> MYARFRTRSKFYFRPARPALAYNVDPNVMRRPKVKRGLLKGTYSDETVDLRDRERLELLESMRHPRERDFYQDHTYHNQWLRRDLEKHQKQQLAARYKYFAPDFEISPWIWYPGDIVEVVSGEGIGQRGTIIAVIKYKNEIVVQNINVQ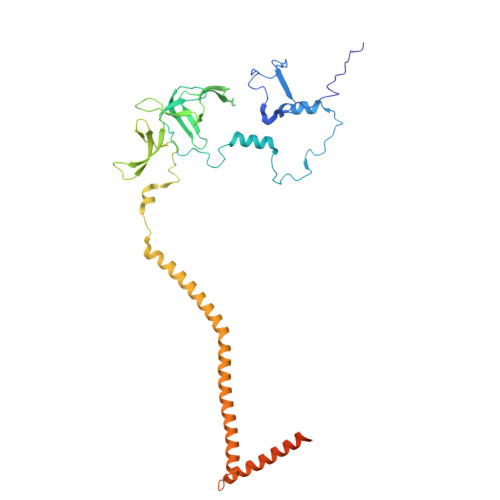DVVIPASESRPEQIVQREHPISVTRVRHVDPSTNEICNIEMVKVRNKETGEMEEKRMSLESGILMSIPPVNDELEVGDPLKDTPIQDADEATYDREAEQAVLVDKRLEAMEEHFVQSLKQSYEFHEPLRRKNAEDMRQFQTDVIDMACAMLGERLLDTVNASDTSSFPAEWQEAIAMHVEEIEAEMEEVAAKEMAEAKEGGAAENEQHDDDLDDDEDELDTSEESVKHV4-HYDROXY-2H-CHROMEN-2-ONE | C9 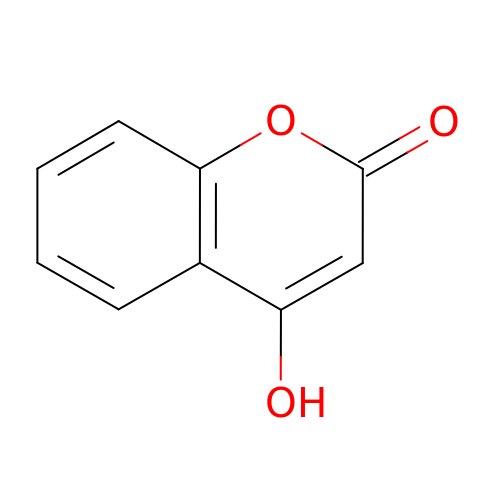H6 O3 | VXIXUWQIVKSKSA-UHFFFAOYSA-N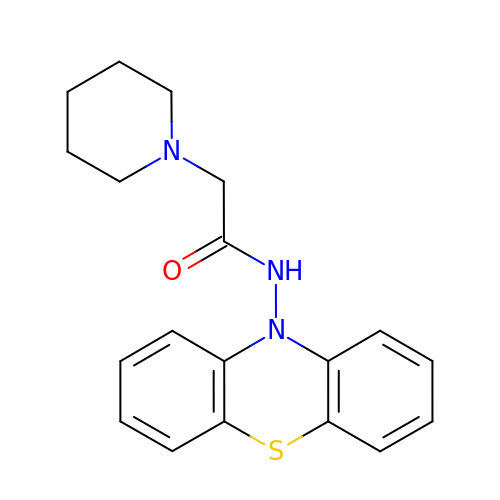N-phenothiazin-10-yl-2-piperidin-1-yl-ethanamide | C19 H21 N3 O S | ALVVXSSFOOYRDP-UHFFFAOYSA-N>[2x]AVSCGQVDTSLTPC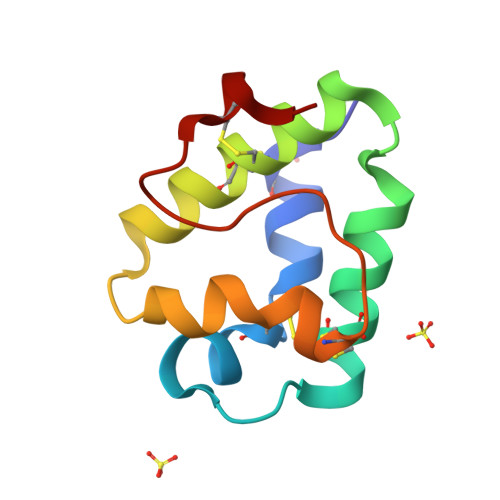LTYLTKGGTPSTQCCSGVRSLKSMTGTKADRQAACNCLKQAAARYQGIKDAAAAALSQKCGVQLSVPISRKTDCSKIS>[2x]MPKRGKKGAVAEDGDELRTEPEAKKS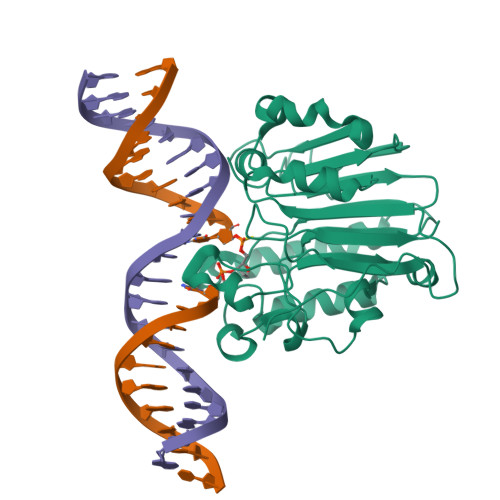KTAAKKNDKEAAGEGPALYEDPPDQKTSPSGKPATLKICSWNVDGLRAWIKKKGLDWVKEEAPDILCLQETKCSENKLPAELQELPGLSHQYWSAPSDKEGYSGVGLLSRQCPLKVSYGIGDEEHDQEGRVIVAEFDSFVLVTAYVPNAGRGLVRLEYRQRWDEAFRKFLKGLASRKPLVLCGDLNVAHEEIDLRNPKGNKKNAGFTPQERQGFGELLQAVPLADSFRHLYPNTPYAYTFWTYMMNARSKNVGWRLDYFLLSHSLLPALCDSKIRSKALGSDHCPITLYLAL7-({[2-hydroxy-1-(hydroxymethyl)ethyl]amino}methyl)-3,5-dihydro-4H-pyrrolo[3,2-d]pyrimidin-4-one | C10 H14 N4 O3 | 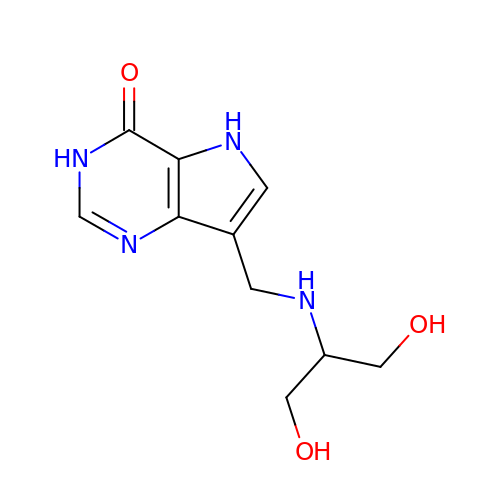YGATXRRSBPFSBK-UHFFFAOYSA-N> GPDSMPDTWNVYDVSQFLRVNDCTAHCDTFSRNKIDGK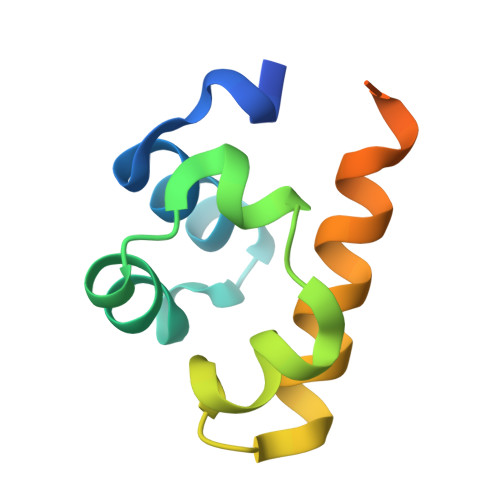RLLQLTKDDIMPLLGMKVGPALKISDLIAQLKCKVNPGRARSHKTNKSPFL>MGTGKGFGVKCVSLKMAKGLTISLLFGWALMAGSSALAATVTDMAGRTVTIPAKVERILLGEGRLFYAVSLLEGNKPLDRIVGWQGDFRKLDPQTYAIYKAKFPQIDQIPLIGNTTADSISPEKVLTLNPDIAIFGLSGHGPGKGSELVKQLEKAGVPVVFVDFRNSPLKNTLPSMRLLGKALHREQQAENYINFYQDNVDKVTDITNKIPEDKKPSVFIELRAGASEECCGTAGKGNMGDFIDQAGGNNIAKNLLPGSLGTVNLEKVLAAKPDIYIASGGKSPGSDAPGVVLGAQVTPEQAQASLQKILGRKGINTLSAVNTGHSYAIWHNYYNSPYNVLAIQSFAKWFYPEQFADLDPKKTMDSLYSQFLAVEPSGTYWIEAKRELDLEHHHHHHHHHH[2x]

Yersinia iron-uptake (Yiu) locus encodes an ABC transporter that is Fur-regulated and has been shown to restore the growth of an enterobactin-deficient mutant strain of Escherichia coli under iron-chelated conditions in vitro. In this report, we document the atomic three-dimensional apo structure of the Yiu SBP YiuA. Structural alignment analysis reveals that YiuA has the greatest degree of structural similarity to cluster A-2 SBPs, which bind chelated metal.

Initially, crystals that grew within three weeks diffracted to approximately 2.20 Å resolution and the Bravais lattice belonged to the orthorhombic crystal system P212121. The YiuA crystals that belonged to this crystal system had unit-cell parameters a = 41, b = 95, c = 172 Å and will be referred to as crystal form 1. In crystal form 1, the two YiuA molecules pack orthogonally in the asymmetric unit with few intermolecular contacts near the base of the amino-terminal lobe of one molecule and the junction between the α-helical backbone and amino-terminal lobe of the other molecule. These intermolecular contacts do not involve helix 5. The final refinement of both YiuA crystal form models revealed several amino-acid Ramachandran outliers. Higher values of each statistic indicate stronger structural similarity and higher quality alignment between the subject and each query. The results from aligning each model with the YiuA crystal form 1 model are summarized in Fig. 2(c), and show that YiuA is most structurally similar to cluster A-2 SBPs and least structurally similar to cluster D-4 SBPs. The total solvent-accessible surface area (SASA) of one molecule in YiuA crystal form 1 is 14 481 Å2 and the cavity SASA is 2682 Å2. Based on these measurements, the dimensions of the YiuA cavity resemble the dimensions of the HmuT cavity, which accommodates a hemin complex, and are considerably larger than the YfeA cavity, which accommodates a metal ion. Atomic distance measurements between the Glu109 and Glu228 C∊ atoms, delineating the base of the cavity, increase from 36.7 Å in crystal form 1 to 40.8 Å in crystal form 2.> GSHMHIKRELWGNLMVAARSNNLEEVKKILKKGIDPTQTNSYHLNRTPLLAAIEGKAYQT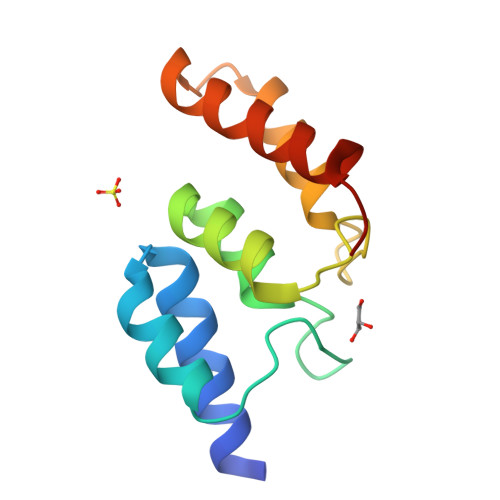ANYLWRKYTFDPNFKDNYGDSPISLLKKQLANPAFKDKEKKQIRALIRGMQEEKIAQSK6-([5-QUINOLYLAMINO]METHYL)-2,4-DIAMINO-5-METHYLPYRIDO[2,3-D]PYRIMIDINE 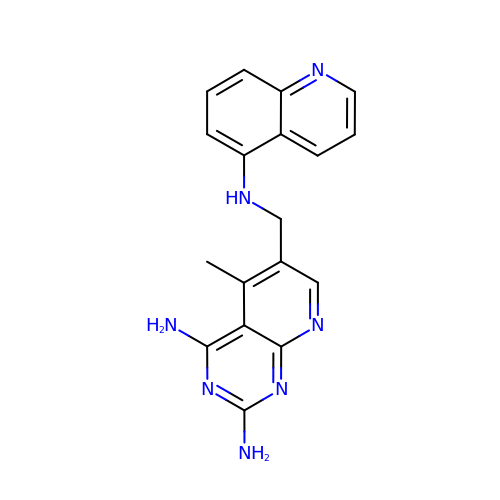| C18 H17 N7 | KMSATRJZEXNGDP-UHFFFAOYSA-N2,4-DIAMINO-5-[3',4'-DIMETHOXY-5'-(5-CARBOXYL-1-PENTYNYL)]BENZYL PYRIMIDINE | C19 H22 N4 O4 | 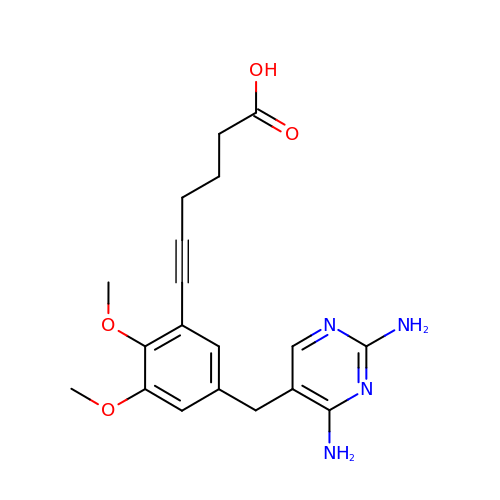JAGSWKLZBKKKJP-UHFFFAOYSA-N> MHHHHHHENLYFQGSHMDATPNAVELTVDNAWFIAETIGAGTFPWVLAITM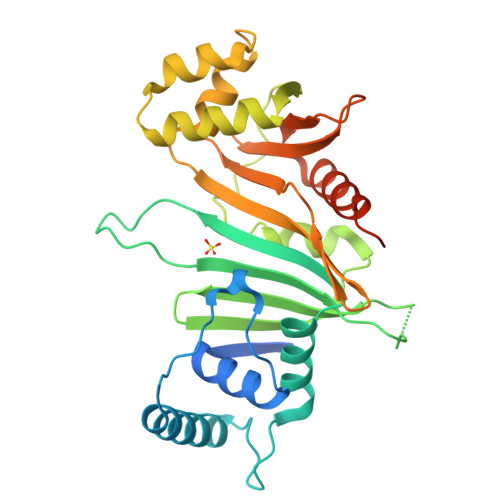PYSDAAQRGAFVDRQRDELTRMGLLSPQGVINPAVADWIKVVCFPDRWLDLRYVGPASADGACELLRGIVALRTGTGKTSNKTGNGVVALRNAQLVTFTAMDIDDPRALVPILGVGLAHRPPARFDEFSLPTRVGARADERLRSGVPLGEVVDYLGIPASARPVVESVFSGPRSYVEIVAGCNRDGRHTTTEVGLSIVDTSAGRVLVSPSRAFDGEWVSTFSPGTPFAIAVAIQTLTACLPDGQWFPGQRVSRDFSTQSS>[4x]XVDSVYRTRSLGVAAEGIPDQYADGEAARVWQLYIGDTRSRTAEYKAWLLGLLRQHGCHRVLDVACGTGVDSIMLVEEGFSVTSVDASDKMLKYALKERWNRRKEPAFDKWVIEEANWLTLDKDVP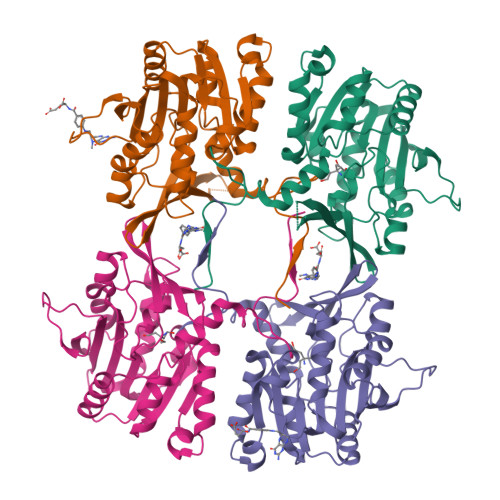AGDGFDAVICLGNSFAHLPDSKGDQSEHRLALKNIASMVRPGGLLVIDHRNYDYILSTGCAPPGKNIYYKSDLTKDITTSVLTVNNKAHMVTLDYTVQVPGAGRDGAPGFSKFRLSYYPHCLASFTELVQEAFGGRCQHSVLGDFKPYRPGQAYVPCYFIHVLKKTG>[5x]GSHMTLTTVIDIGNFSTKYAYKDAAQIKVGSFPSILHSYKPLEDYEGMERVEYNGLDYYVGETVKNFYFGREEQMYFGNTRKGHMEGQIRLVYALYTIFKETGAAEFNLILTCPYESMVTDKKYFVQHFEGEREVIVEGKSFKFTVHNIVMAAEGLGALNFSDSLNCVIVDAGSKTL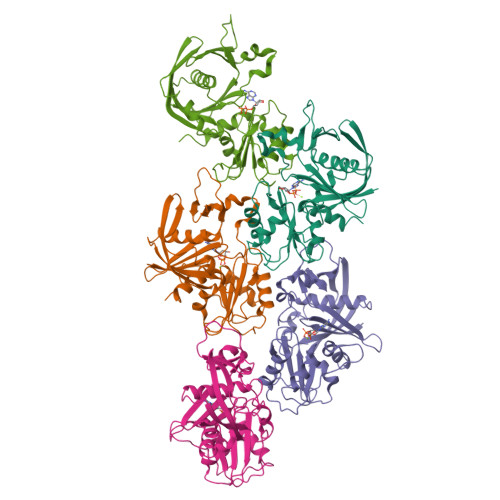NVLYLINGSISKMDSHTINGGTIDNSIMDLAKTFAKTCSNIDYDYPIVCTGGKAEEMKECLENVGYSTVSSAELGEDKPSYYVNSVGLLLKYGRKFEEMFA>HHHHHHMDLVEKVKELCLELEEENLAKAIERFITLTHGIEKTRGEAFAKASIYGFLEGILTTLKMKYSNEKIET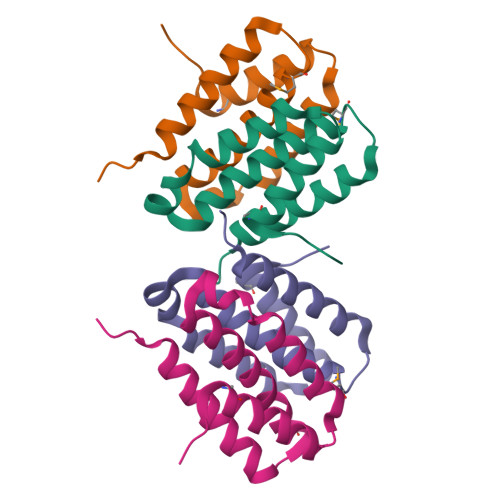LLNEVKTAREETEALLRKPRPPLLVDNDL[4x]> MTPESVMMMGTEAMKVALALAAPLLLVALITGLIISILQAATQINEMTLSFIPKIVAVFIAIIV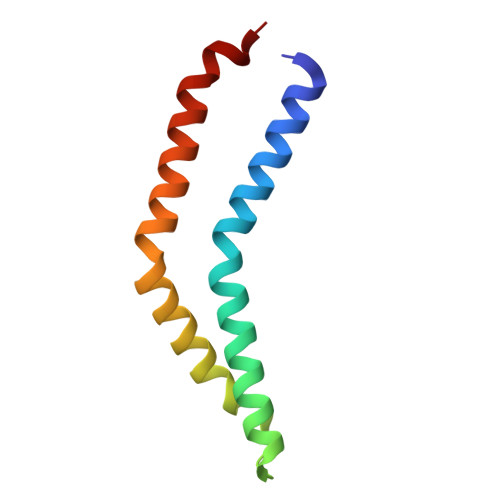AGPWMLNLLLDYVRTLFSNLPYIIG> AGVGTVPMTDYGNDIEYYGQVTIGTPGKKFNLDFDTGSSDLWIASTLCTNCGSRQTKYDPNQSSTYQADGRTWSISYGDGSSASGILAKDNVNLGGLLIKGQTIELAKREAASFASGPNDGLLGLGFDTITTVRGVKTPMDNLISQGLISRP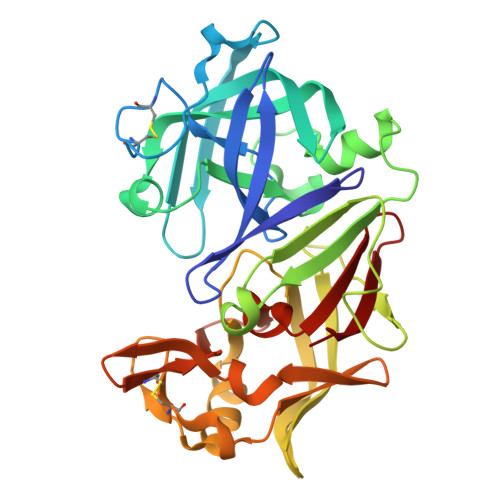IFGVYLGKAKNGGGGEYIFGGYDSTKFKGSLTTVPIDNSRGWWGITVDRATVGTSTVASSFDGILDTGTTLLILPNNIAASVARAYGASDNGDGTYTISCDTSRFKPLVFSINGASFQVSPDSLVFEEFQGQCIAGFGYGNWDFAIIGDTFLKNNYVVFNQGVPEVQIAPVAE>[2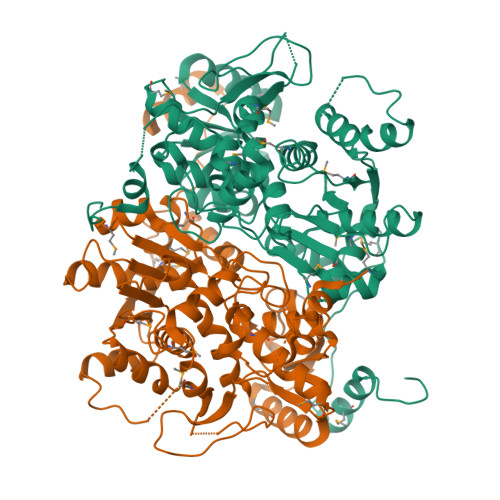x]ADGNNIKAPIETAVKPPHRTEDNIRDEARRNRSNAVNPFSAKYVPFNAAPGSTESYSLDEIVYRSRSGGLLDVEHDMEALKRFDGAYWRDLFDSRVGKSTWPYGSGVWSKKEWVLPEIDDDDIVSAFEGNSNLFWAERFGKQFLGMNDLWVKHCGISHTGSFKDLGMTVLVSQVNRLRKMKRPVVGVGCASTGDTSAALSAYCASAGIPSIVFLPANKISMAQLVQPIANGAFVLSIDTDFDGCMKLIREITAELPIYLANSLNSLRLEGQKTAAIEILQQFDWQVPDWVIVPGGNLGNIYAFYKGFKMCQELGLVDRIPRMVCAQAANANPLYLHYKSGWKDFKPMTASTTFASAIQIGDPVSIDRAVYALKKCNGIVEEATEEELMDAMAQADSTGMFICPHTGVALTALFKLRNQGVIAPTDRTVVVSTAHGLKFTQSKIDYHSNAIPDMACRFSNPPVDVKADFGAVMDVLKSYLGSNTLTS>[2x]MASTDYHVDLTNCDREPIHIPGYIQPHGCLIACDNAMRMVLRHSENCGELLGLEGDLNGRTAEDVLGKRLVHDLRNALTVTGKTTRPAMLPAMETSDGRSFDISLHRYKSTTIIEFEPSDSDTQPLGTARKMVDRIREADSVESLISRTTRLVKATLGYDRVLIYRFEEDGAGKVVSEAKQPELESFLGQYFPASDIPQQARALYLKNTLRIISDASGTPIPVLPAVDVSGEPLDLSYAHLRNFSPIHCEYLRNMGVAASMSISVIVDDALWGLIVCHHCSPRVLSMPVRIAAAMFGEFFSMFLQVLKQKRRLDTINHAHAALDRFLRLAAHRANLEELLVDSFQDFARLIPCDGVGLWVGNNWHGHGATPPHDAIPRLARFVASVSEGRVWATHALSQAIPEAEIYADTAAGMLAIPISQVKSDYLLFFRKEIVQNLNWAGNPEKSYETGPMGDRLTPRKSFAIWKESVRLQAQPWSEADREIAETARIALVGVAFHHSELMAGLEYK

Phytochromes are biliproteins of plants, bacteria and fungi that use red light as a source of information to regulate fundamental physiological processes, such as photosynthesis, seed germination, flowering and shade avoidance. The molecular architecture of phytochromes shares a common photosensory core module (PCM), which is composed of PAS (Per/Arnt/Sim), GAF (cGMP phosphodiesterase/adenyl cyclase/FhlA) and PHY (phytochrome-specific) domain4–6. Bacterial phytochromes can be grouped into prototypical and bathy phytochromes, in which the red-absorbing Pr and far-red-absorbing Pfr are the thermodynamically stable states, respectively. The conjugate Meta-F and Pfr crystal structures has been obtained from the engineered photoactivatable near-IR fluorescent protein (Agp2-PAiRFP2), derived from the bathy phytochrome Agp2 from Agrobacterium fabrum.

Here we describe the crystal structure of a Meta-F intermediate of the PCM of a bathy phytochrome at 2.16 Å resolution formed during the Pfr→Pr phototransformation. The intermediate has been generated by irradiating crystals of the parent Pfr state at ambient temperature and identified as Meta-F by resonance Raman (RR) spectroscopy. The asymmetric unit includes two molecules (Mol A and B), which differ in terms of the intermolecular interactions of their N-termini. Compared to the Pfr structure, the overall fold of the protein and specifically the α-helical segment of the tongue remained unchanged but significant structural changes were observed for the chromophore and its binding pocket as reflected by the ΔFo (FoMeta-F−FoPfr) electron density maps. The C-D methine bridge has undergone the expected E→Z isomerization as also shown by 2mFo-DFc and several types of omit electron density maps. The resulting ZZZssa stereochemistry of the chromophore structure exhibits a deviation of the tilt angle between neighbouring C and D pyrrole rings (38.9° and 44.5° for Mol A and Mol B, respectively). The first group includes a rearrangement of the extended hydrogen bond network surrounding the chromophore, most likely initiated by the almost 180° rotation of ring D and facilitated by conformational changes of the participating amino acid residues and movements of ordered water molecules. In the structure of the Meta-F sub-states of Mol A and Mol B, these Pr characteristic features including the concomitant re-positioning of Trp440 away from the sterically pressing Gln190 were not visible. Instead, the amino acid segments 439–448 in Mol A and 439–442 in Mol B were not resolved in the electron density map, indicating a disordering of the polypeptide backbone.> GSGGSHMGSGRIELNSVSFRYNGDYVLKDVNAEFETGKIYVVVGKNGSGKTTLLKILAGLLAAAG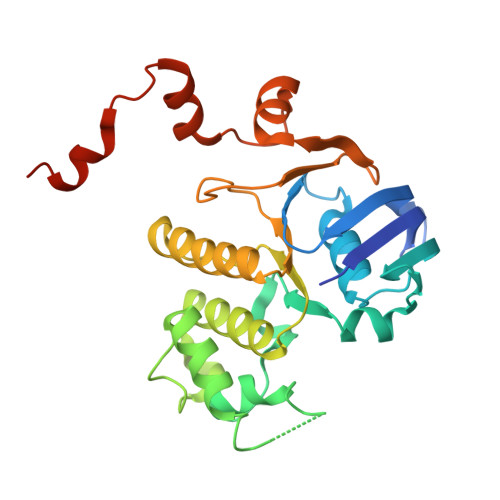EIFLDGSPADPFLLRKNVGYVFQNPSSQIIGATVEEDVAFSLEIMGLDESEMRKRIKKVLELVGLSGLAAADPLNLSGGQKQRLAIASMLARDTRFLALDEPVSMLDPPSQREIFQVLESLKNEGKGIILVTHELEYLDDMDFILHISNGTIDFCGSWEEFVEREFDDVEIPFKWKLWKKCGKINLWEDRYENSGNQRRRDTV>[2x]TDKRKDGSGK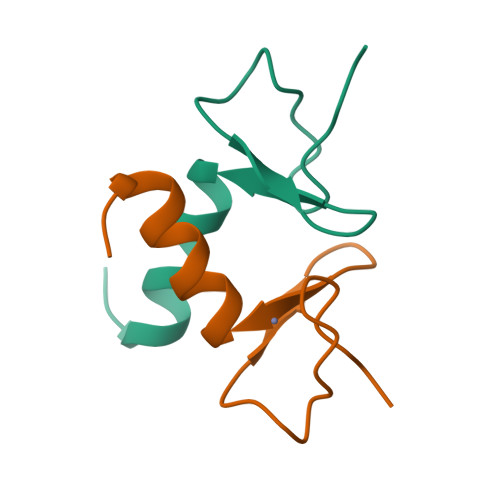LLYCSFCGKSQHEVRKLIAGPSVYICDECVDLCNDIIREEI> GQS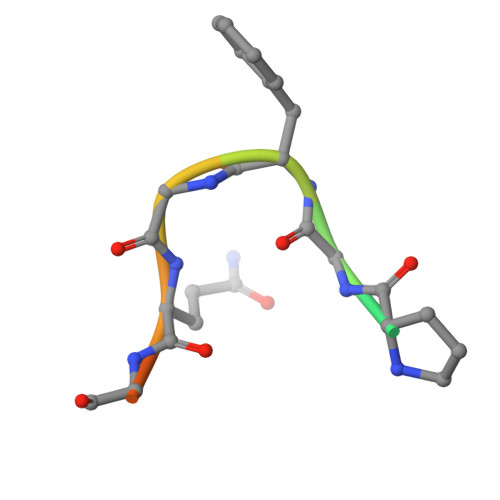PGFGQGGSV> MPFVNKQFNYKDPVNGVDIAYIKIPNAGQMQPVKAFKIHNKIWVIPERDTFTNPEEGDLNPPPEAKQVPVSYYDSTYLSTDNEKDNYLKGVTKLFERIYSTDLGRMLLTSIVRGIPFWGGSTIDTELKVIDTNCINVIQPDGSYRSEELNLVIIGPSADIIQFECKSFGHEVLNLTRNGYGSTQYIRFSPD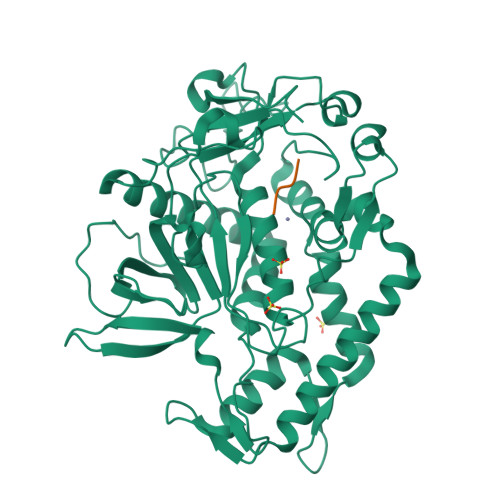FTFGFEESLEVDTNPLLGAGKFATDPAVTLAHELIHAGHRLYGIAINPNRVFKVNTNAYYEMSGLEVSFEELRTFGGHDAKFIDSLQENEFRLYYYNKFKDIASTLNKAKSIVGTTASLQYMKNVFKEKYLLSEDTSGKFSVDKLKFDKLYKMLTEIYTEDNFVKFFKVLNRKTYLNFDKAVFKINIVPKVNYTIYDGFNLRNTNLAANFNGQNTEINNMNFTKLKNFTGLFELEHHHHHH;> RRGLX> MLRTCRVLRFRMKLGSMYVDYKIVSRNHRRSIRVEDALVDPLLPTTVVPLHWLEQLRCPSTRLLTGYH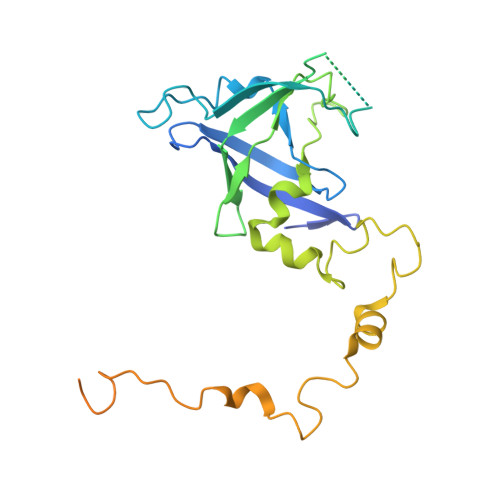TEEAVYAKPNYGDRVSRTPALLSLPDAAAKTADNGAHANAIRAGPVVLYITGQSIPVVLNPLFVQPDEWGLTQSNGEWDLRIGMDAIEQCSLYAELRPGGLLYSKLPHASLTEAMEPVQDTLKRYGMRCALAESPLVPRPWTRMRYMFIDELQRGQKMTEFVGYNPRNGTQWRFSQHTKYFRTGIWRETIRRNEMNDGLHAHSSWQKSPQQAVPEISFLAPYP Clostridioides difficile causes life-threatening gastrointestinal infections. Herein, we report 30 X-ray structures from a structure genomics pipeline spanning 13 years, representing 10.2% of the X-ray structures for this important pathogen. The Center for Structural Biology of Infectious Diseases (CSBID, formerly the Center for Structural Genomics of Infectious Diseases) implemented a structural biology pipeline starting in 2010 through paired efforts with systems biology, bioinformatics, and other research specialists in C. difficile pathogenesis. This project ultimately involved 335 proteins linked with pathogenesis, metabolism, and antimicrobial resistance.

The structures presented here are part of the C. difficile 630, R20291, and Y384 sets nominated at CSBID. The overall success of structure determination for C. difficile in both CSBID pipelines was 7%, with a total of 23 unique structures and eight variants or ligand-bound proteins determined.

>[4x]MVDYSDCFEGISGGAIFYNTKNKEYNIYNKELIETRRSPCSTFAIVSTLIGLEKGVINSKESVMGYDGTEYPNKNWNKNLSLEEAFKESCVWYYKKLIDKVDAKSVQNILDDLKYGNCDISEWEGDLKNGKGHLNGFWLESSLQISPKEQVQTMAKIFEGDTNFKKEHINILRDIMKIDVNDKNINVYGKTGTGFDEKNKRVDAWFVGMLEREGDTYYFAIKSDDSNKEITGPKVKEIAINIIKKYYSVREGAAL>[9x]MTVGTLVASVLPATVFEDLAYAELYSDPPGLTPLPEEAPLIARSVAKRRNEFITVRHCARIALDQLGVPPAPILKGD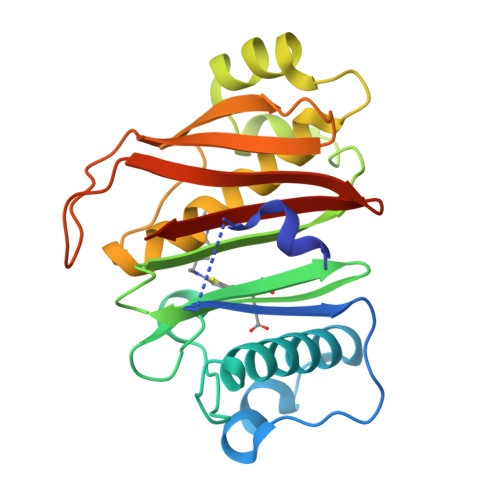KGEPCWPDGMVGSLTHCAGYRGAVVGRRDAVRSVGIDAEPHDVLPNGVLDAISLPAERADMPRTMPAALHWDRILFCAKEATYKAWFPLTKRWLGFEDAHITFETDSTGWTGRFVSRILIDGSTLSGPPLTTLRGRWSVERGLVLTAIVLAGENLYFQ>MGSKRRFSSEHPDPVETSIPEQAAEIAEELSKQHPLPSEEPLVHHDAGEFKGLQRHHTSAEEAQKLEDGKINPFTGREFTPKYVDILKIRRELPVHAQRDEFLKLYQNNQIMVFVGETGSGKTTQIPQFVLFDEMPHLENTQVACTQPRRVAAMSVAQRVAEEMDVKLGEEVGYSIRFENKTSNKTILKYMTDGMLLREAMEDHDLSRYSCIILDEAHERTLATDILMGLLKQVVKRRPDLKIIIMSATLDAEKFQRYFNDAPLLAVPGRTYPVELYYTPEFQRDYLDSAIRTVLQIH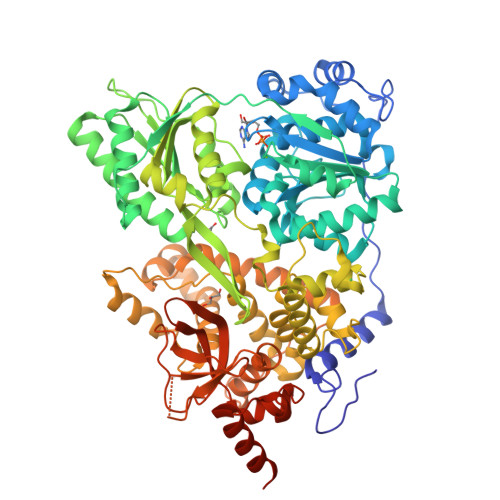ATEEAGDILLFLTGEDEIEDAVRKISLEGDQLVREEGCGPLSVYPLYGSLPPHQQQRIFEPAPESHNGRPGRKVVISTNIAETSLTIDGIVYVVDPGFSKQKVYNPRIRVESLLVSPISKASAQQRAGRAGRTRPGKCFRLYTEEAFQKELIEQSYPEILRSNLSSTVLELKKLGIDDLVHFDFMDPPAPETMMRALEELNYLACLDDEGNLTPLGRLASQFPLDPMLAVMLIGSFEFQCSQEILTIVAMLSVPNVFIRPTKDKKRADDAKNIFAHPDGDHITLLNVYHAFKSDEAYEYGIHKWCRDHYLNYRSLSAADNIRSQLERLMNRYNLELNTTDYESPKYFDNIRKALASGFFMQVAKKRSGAKGYITVKDNQDVLIHPSTVLGHDAEWVIYNEFVLTSKNYIRTVTSVRPEWLIEIAPAYYDLSNFQKGDVKLSLERIKEKVDRLNELKQGKNKKKSKHSKKHHHHHH[2x]> SVCAAQNCQRPCKDKVDWVQCDGGCDEWFHQVCVGVSPEMAENEDYICINCA;> ART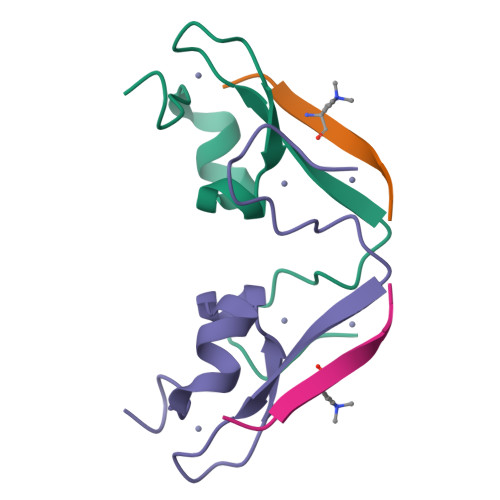KQTARK4-[5-(7-fluoranylquinolin-4-yl)-1-methyl-imidazol-4-yl]-3,5-dimethyl-1,2-oxazole | C18 H15 F N4 O | 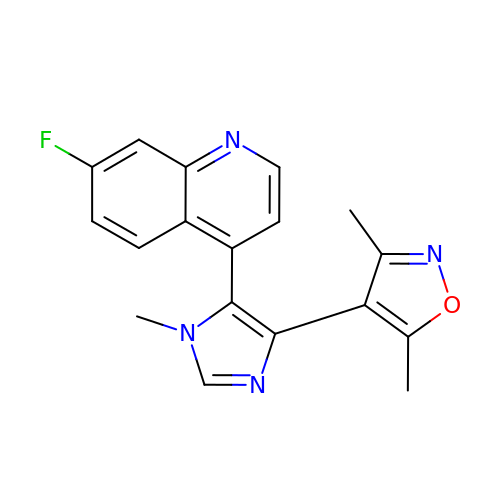FOQLCYIBXICLES-UHFFFAOYSA-N>MKLNIRAQTAQNQHNNSPIVLVHGLFGSLDNLGVLARDLVNDHNIIQVDVRNHGLSPREPVMNYPAMAQDLVDTLDALQIDKATFIGHSMGGKAVMALTALAPDRIDKLVAIDIAPVDYHVRRHDEIFAAINAVSESDAQTRQQAAAIMRQHLNEEGVIQFLLKSFVDGEWRFNVPVLWDQYPHIVGWEKIPA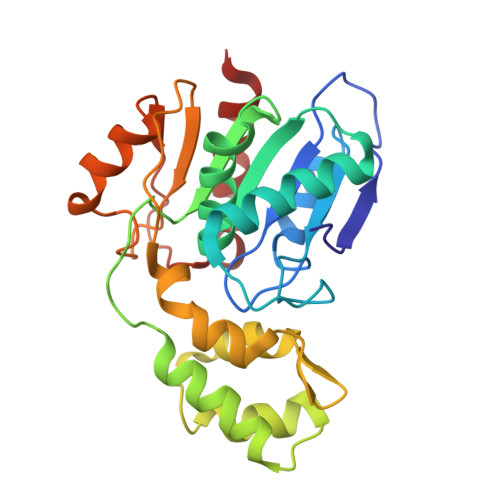WDHPALFIPGGNSPYVSEQYRDDLLAQFPQARAHVIAGAGHWVHAEKPDAVLRAIRRYLNDH[2x]>[4x]GSKGRLVIYCSATNVMCENAAKTFEQKYDVKTSFIRNGSGSTFAKIEAEKNNPQADVWYGGTLDPQSQAGELGLLEAYRSPNIDQIMPKFQDPAKVKGNLSSAVYIGILGFAVNTERLKKLGIEKIPQCWNDLTDPKLKGEIQIADPQSSGTAYTAIATFAQLWGEDKAFDYFKHLHPNISQYTKSGITPARNAARGETTVGIGFLHDYALEKEQGAPLEMVVPCEGTGY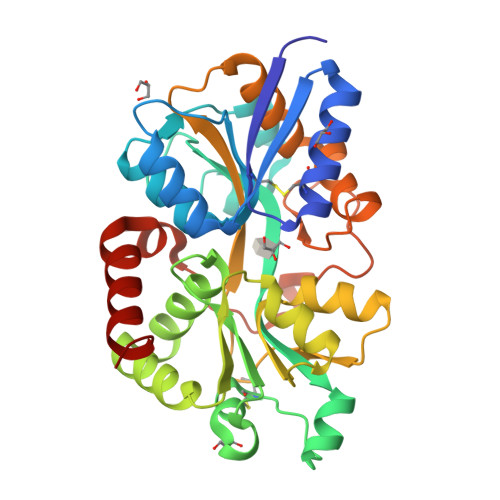ELGGVSILKGARNLDNAKLFVDFALSKEGQETAWKKGQALQTLTNTTAEQSPLAFDLTKLKLIDYDFEKYGASDERKRLINKWVDEIKLAK> MSQEKKAKKIILHYPDDTPAGYIEYAEGSSSIYDNEGNFLFKVEGKFPPQPKKSSDYSWIEKVLEMGLQDSRKRFILYVASRYLVNVKGVNEDEALQTLKEFYYKLQSGKVYESWLKSVINGVKKKGLLPWSLKRIEERDKEM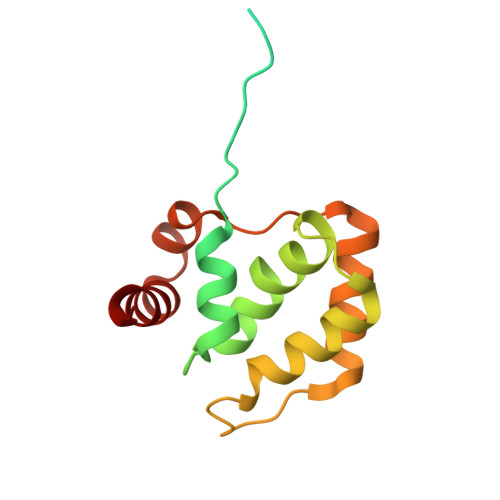YNEIIRVLKNS> GPH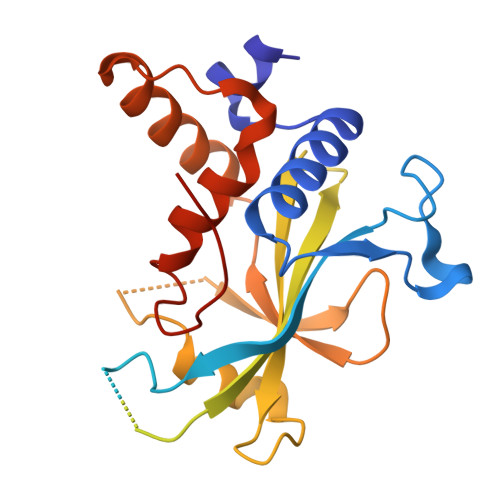MAFKEKGVLSVSEFVLAGDNLVSKCPTWSWESGDASKRKPYLPSDKQFLITRNVPCLRRAASVAEDYEAAGGEVLVDDEDNDGWLATHGKPKDKGKEEDNLPSMDALDINEKNTIQSIPTYFGGEEDDDIPDMEEFDEADNVVENDPATLQSTYLVAHEPDDDNILRTRTYDLSITYDKYYQTPRVWLTGYDESRMLLQPELVMEDVSQDHARKTVTIEDHPHLPGKHASVHPCRHGAVMKKIIDVLMSRGVEPEVDKYLFLFLKFMASVIPTIEYDYTMDFDLGSSST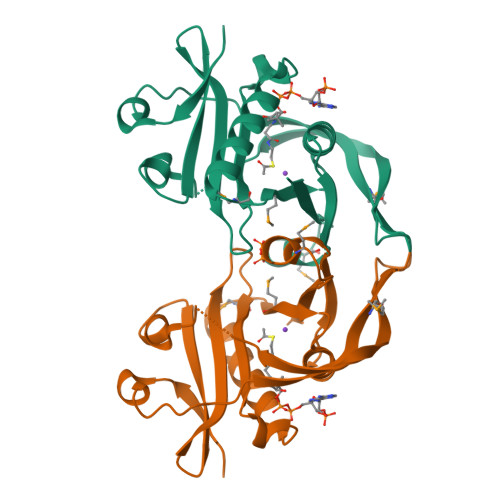>SNAMSLLIRELETNDLDNFPEIDDSFIVNARLMLSLSKVNRRIEYTVEDVPSYEKSYLQNDNEELVYNEYINKPNQIIYIALLHNQIIGFIVLKKNWNNYAYIEDITVDKKYRTLGVGKRLIAQAKQWAKEGNMPGIMLETQNNNVAACKFYEKCGFVIGGFDFLVYKGLNMTSDEVAIYWYLHFDS[3x]>[8x]MGVVPQYGGGGNHGGGGNNSGPNSELNIYQYGGGNSALALQTDCRNSDLTITQH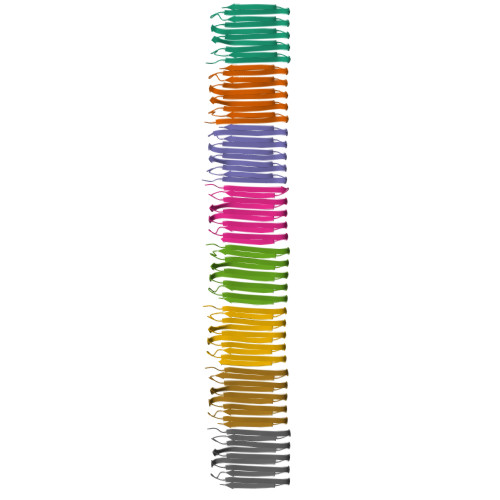GGGNGADVGQGSDDSSIDLTQRGFGNSATLDQWNGKNSEMTVKQFGGGNGAAVDQTASNSSVNVTQCGFGNNATAHQYHHHHHH>[2x]GSPGIPGSTRMAYQHCPFDTLLILDFETTSDAANQDYPCEVIQFAIVAYDVPNDKIREDISFNKYVKPVLNRTLTKNCVDFTGIPQRSIDTADTFDVVYEQFQQWLITLGLEEGKFAFVCDSRQDLWRI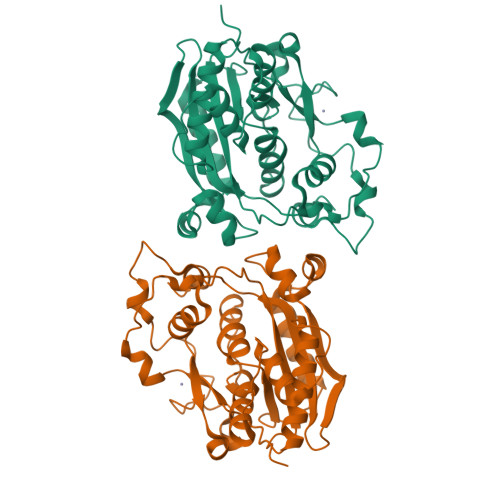AQYQMKLSNIQMPAFFRQYINLYKIFTNEMDRMGPKELSATTNIGKMNEYYDLPTIGRAHDAMDDCLNIATILQRMINMGAKVTVNELLTCCASWRRQPLVYNKEWRSSFMDAGKIFERVLPLVVTTIRAGDFRLEMYGVCRYCRKGMDVCGTSHQQTPHDLYKNEEDPIHFAKIAGYY>SMDDSEKDFNLKVVLVSFKQCLTDKGEVLLDHYIAGWKGLVRFLNSLGAVFSFISKDVVAKLQIMERLRSSPQSEHYTSLQSMVAYEVSNKLVDMDHRSHPRHPHSGCRTVLRLHRALHWLQLFLDGLRTSSEDARTSTLCSEAYN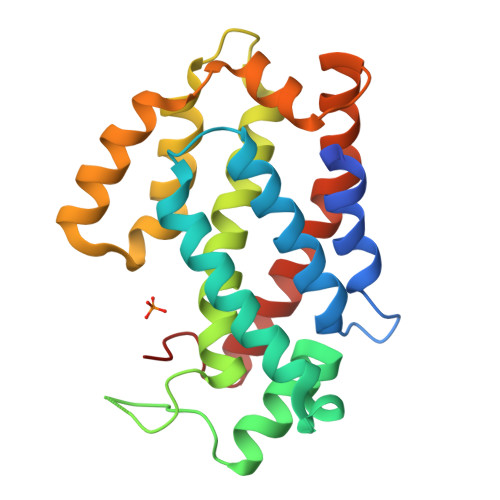ATLANYHSWIVRQAVTVAFCALPSRKVFLEAMNMESTEQAVEMLGEALPFIEHVYDISQKLYAEHSLLDLP[8x]> MFKFDKKQEVFELGGVKFGGQPGENPTVLVSTMFYARHKIVTDEDKGIFDRAAAETLWNTQVSLSDATGLPYVNQIVGETPESIKRYIEWFVGIDDRTPFLIDSSAGNVRAAAAQYCTEIGVADRAIHNSINASIEQSEIDVLTESDVSAAIVLAFNATDPTVKGKIDILEVGGSGQTK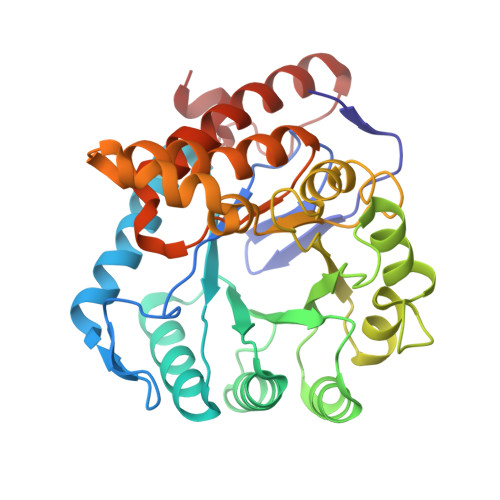GMLQVAKECGIKYPIIDVAAMPLGAGSGATIRSVPTLKGKFGLPIGGGYHNMASAWDWLRKFKKTQPDPKAIYMPTDIGTNLVAQIAGSDYLLYGPIENVNQIFPAVAMVDIMLGETAKELGVEIADLENHPVTKLT9H-purine-6-thiol 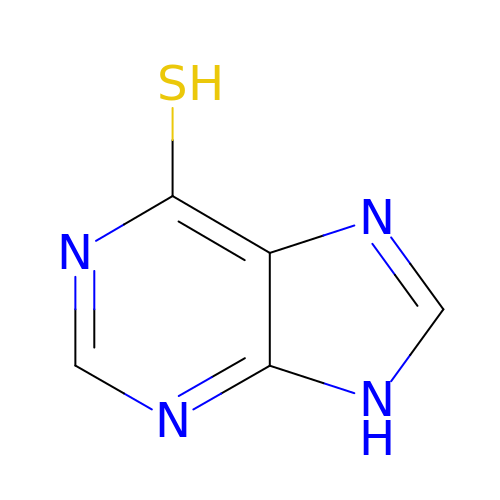| C5 H4 N4 S | GLVAUDGFNGKCSF-UHFFFAOYSA-N> GDKLLSVCMNSKRHKQEPGPEDELYQECRPWEDNACCTRSTSWEAHLEEPLLFDFSMMHCGLLTPACRKHFIQAICFHECSPNLGPWIQPVVPNGQEEQRVWGVPLCQEDCEDWWRACHSSLT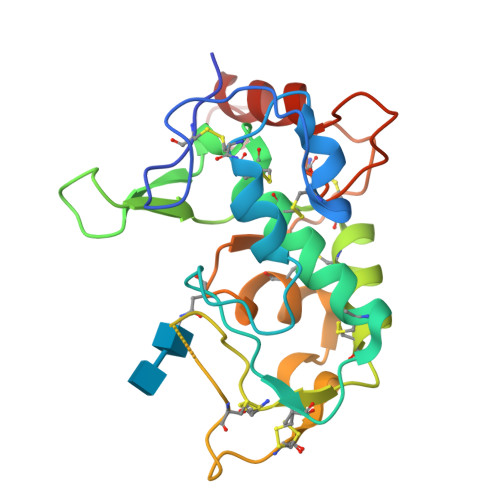CKSNWLHGWDWSEEKKHCPAHEPCLPFSYHFPTPDDLCEKIWNNTFKASPERRNSGRCLQKWFEPTLSNPNVEVALHFASGLEVLFQ>MLYLVRMTVNLPRNLDPREEERLKASAKARSRTLQEQGQWRYLWRTTGKYGNISVF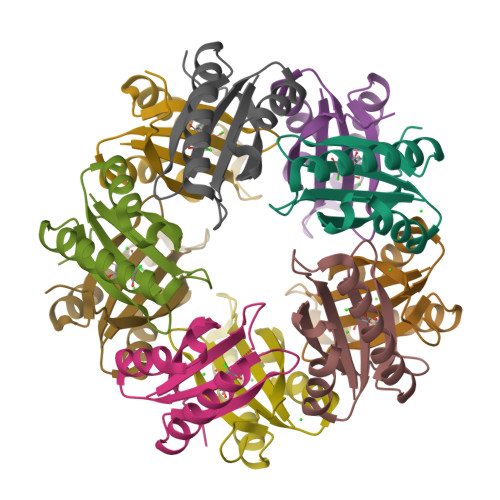DVNSHDELHEILWSLPFFPYLTIDVEPLSHHPARVGKD[10x]>MTDMSIKFELIDVPIPQGTNVIIGQAH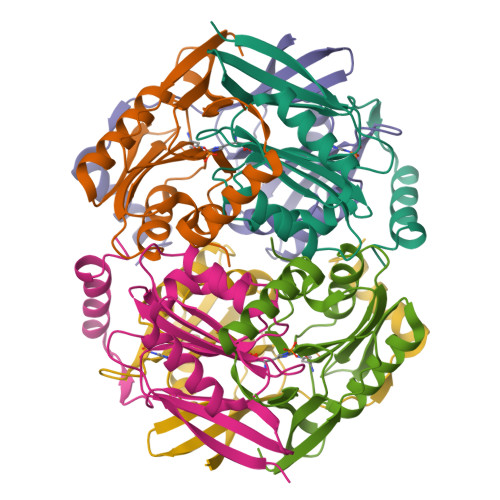FIKTVEDLYEALVTSVPGVKFGIAFCEASGKRLVRHEANDEELRNLAIDLCKKIAAGHVFVIYIRNAWPINVLNAIKNVPEVVRIFAATANPLKVIVAEVEPERRGVVGVVDGHSPLGVETEKDREERKKFLREVVKYKL[3x]>MDIAKRCESNPLLSPKDLKAGINDMEITCLLNPGVFKFKGKTWLLLRVAERPVQQEGIISFPIYDEQGQIKVMSFAENDPDLDASDPRVIGYKGKNYLTTMSYLRLVSSEDGIHFHDEPGYPPIFGKGELEAFGIEDCRVASTKDGFYLTFTEVSSVAVGVGMMHTNDWKTFEHYGMILPPHNKDCALFEEKINDKYYTFHRPSSPELGGNYIWLAESPDLRHWGNHKCVATTRDGFWDCARVGAGAAPIKTEAGWLEIYHGAD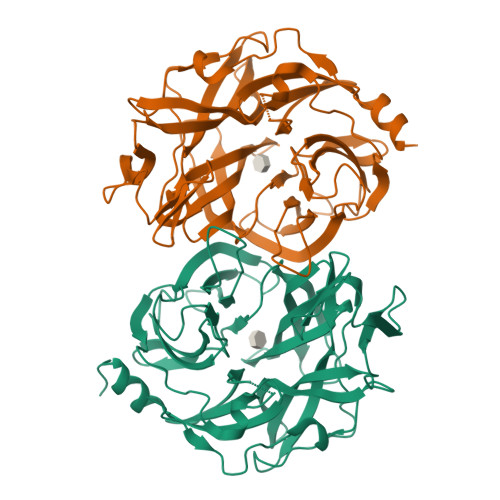FNHRYCLGALLLDLNDPSKVLARSKEPIMEPIASYEQTGFFGNVIFTNGQLVDGDTITIYYGASDEVICKAELSVKEILNILNVGIL[2x]>[2x]RSHHHHHHSSGPTAIESCMVKFELSSSKWHMTSPKPHCVNTTSDGKLKILQSG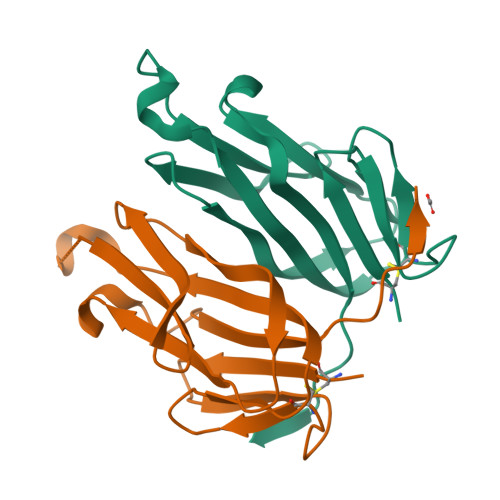TYLIYGQVIPVDKKYIKDNAPFVVQIYKKNDVLQTLMNDFQILPIGGVYELHAGDNIYLKFNSKDHIQKTNTYWGIILMPDLPFIS> ANSTAELEELLMQRSLTDPQLQAAAAAAADFRILPDATVIKIGGQSVID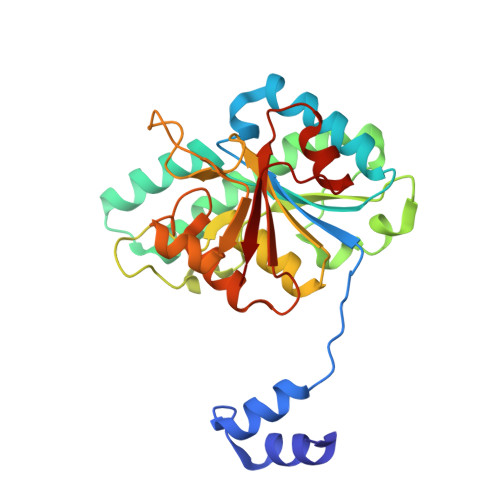RGRAAVYPLVDEIVAARKNHKLLIGTGAGTRARHLYSIAAGLGLPAGVLAQLGSSVADQNAAMLGQLLAKHGIPVVGGAGHSAVPLSLAEVNAVVFSGMPPYKLWMRPAAEGVIPPYRTDAGCFLLAEQFGCKQMIFVKDEDGLYTANPKTSKDATFIPRISVDEMKAKGLHDSILEFPVLDLLQSAQHVREVQVVNGLVPGNLTRALAGEHVGTIITAS>[2x]MGSSHHHHHHSSGENLYFQHMGLLSTNFDMIQALPLNVKQRVCALKNLQMKTIQIESDFYKRVHELEIEFEGKFKSTFDQRKAIVAGEVEPTKEQIDTPILEGLEGDQLAELYKAAEADPSAKGIKDFWLTALRTHDLVAEAIEEHDVPIL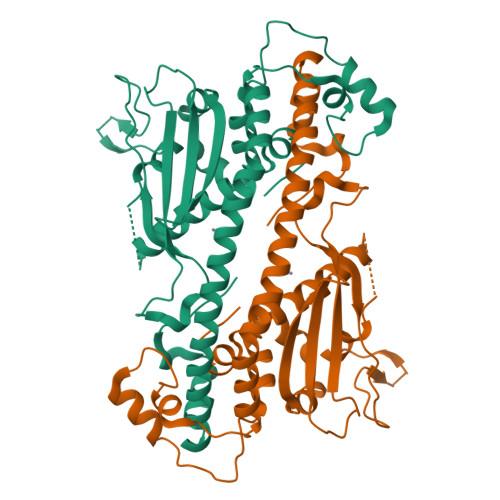SYLTDVTTAASKDPAGFKIEFHFATNPYFKNQVLTKTYLLGFDPDAEAPLQFDGPHVIRAVGDTIEWEDGKNVTKKAVKKKQKKGANAGKFLTKTVKADSFFNFFEPPKSKDERNEDEDDEQAEEFLELDYEMGQAIRDTIIPRAVLFYTGELQSDD>SNAMNKVITDLDKALSALKDGDTILVGGFGLCGIPEYAIDYIYKKGIKDLIVVSNNCGVDDFGLGILLEKKQIKKIIASYVGENKIFESQMLNGEIEVVLTPQGTLAENLHAGGAGIPAYYTPTGVGTLIAQGKESREFNGKEYILERAITGDYGLIKAYKSDTLGNLVFRKTARNFNPLCAMAAKICVAEV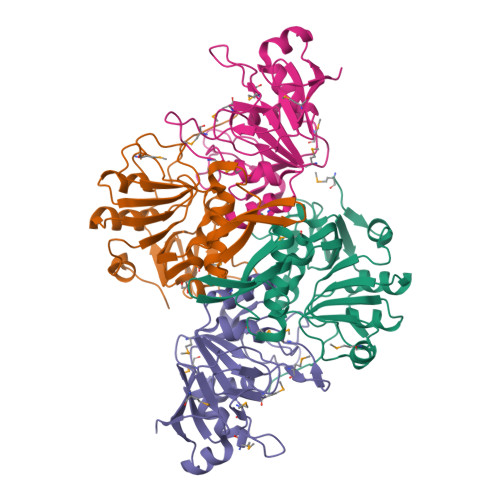EEIVPAGELDPDEIHLPGIYVQHIYKGEKFEKRIEKITTRSTK[2x];>[2x]MREAIIKRAAKELKEGMYVNLGIGLPTLVANEVSGMNIVFQSENGLLGIGAYPLEGSVDADLINAGKETITVVPGASFFNSADSFAMIRGGHIDLAILGGMEVSQNGDLANWMIPKKLIKGMGGAMDLVHGAKKVIVIMEHCNKYGESKVKKECSLPLTGKGVVHQLITDLAVFEFSNNAMKLVELQEGVSLDQVKEKTEAEFEVRL>[4x]MNSTAQGQLKSIIERVERLEVEKAEIMEQIKEVYAEAKGN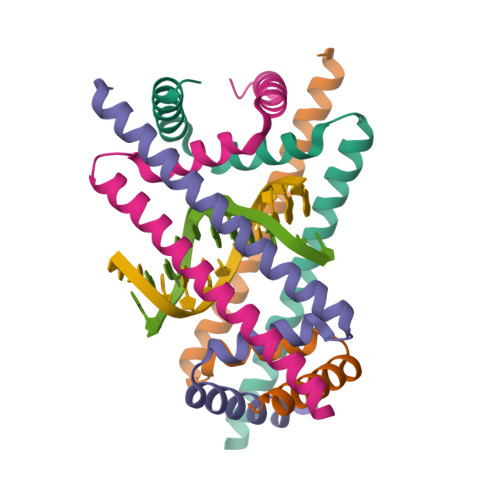GFDVKVLKKVVRIRKQDRAKRQEEDAILDLYMSAIGEI>[2x]MNDIVASTQLPNTIKTITNDLRKLGLKKGMTVIVHSSLSSIGWISGGAVAVVEALMEVITEEGTIIMPTQSSDLSDPKHWSRPPVPEEWWQIIRDNVPAFEPHITPTRAMGKVVECFRTYPNVVRSNHPLGSFAAWGRHAEEITVNQSLSMSLGEESPLRKIYDLDGYILLIGVGYDSNTSVHLSEVRSGACELIKVGAPIIENGERVWKEFVDMDYDSDKFVEIGVEFEQKGTVT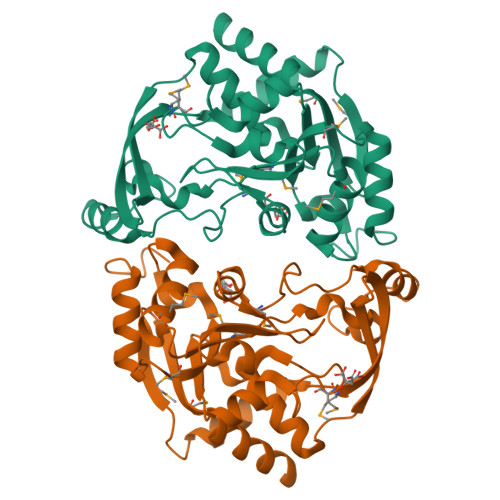MGKIGNAKCRLMKQRDIVDFGTEWFRKKN>[3x]MGSSHHHHHSSG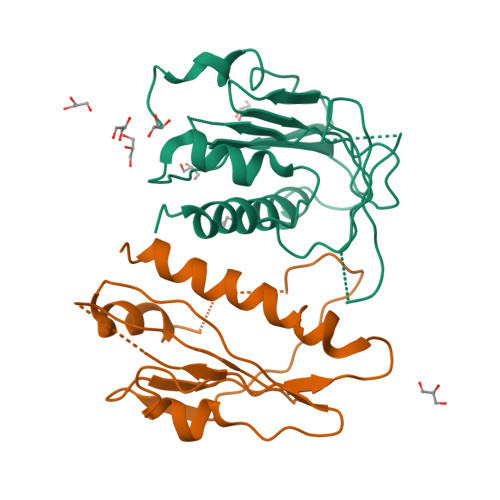ENLYFQGHMRSPVQLQHGSDATNGFHTLQPHDQTDGPIKRVCLTRGMHVPEHVAMHHTHDVGPDQCCSSVVQMIHAPPESVWALVRRFDNPKVYKNFIRQCRIVQGDGLHVGDLREVMVVSGLPAVSSTERLEILDEERHVISFSVVGGDHRLKNYRSVTTLHASDDEGTVVVESYIVDVPPGNTEEETLSFVDTIVRCNLQSLARSTNRQ> LPDSVDWREK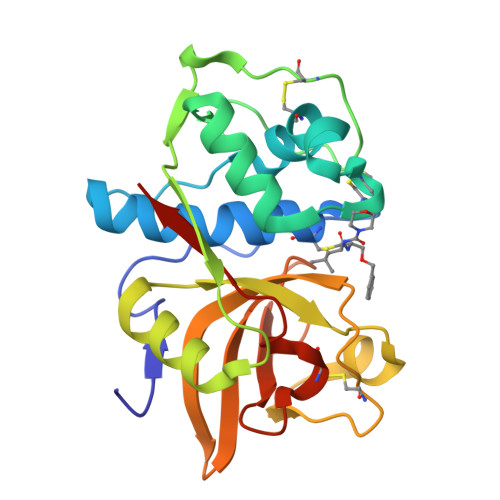GCVTEVKYQGSCGACWAFSAVGALEAQLKLKTGKLVSLSAQNLVDCSTEKYGNKGCNGGFMTTAFQYIIDNKGIDSDASYPYKAMDQKCQYDSKYRAATCSKYTELPYGREDVLKEAVANKGPVSVGVDARHPSFFLYRSGVYYEPSCTQNVNHGVLVVGYGDLNGKEYWLVKNSWGHNFGEEGYIRMARNKGNHCGIASFPSYPEIHHHHH>[2x]MKLYVFLVNTGTTLTFDTELTVQTVADLKHAIQSKYKIAIQHQVLVVNGGECMAADRRVCTYSAGTDTNPIFLFNKEMILCDRPPAIPKTTFSTENDMEIKVEESLMMPAVFHTVASRTQLALEMYEVAKKLCSFCEGLVHDEHLQHQGWAAIMANLEDCSNSYQKLLFKFESIYSNYLQSIEDIKLKLTHLGTAVSVMAKIPLLECLTRHSYRECLGRLDSLPEHEDSEKAEMKRSTELVLSPDMPRTTNESLLTSFPKSVEHVSPDTADAESGKEIRESCQSTVHQQDETTIDTKDGDLPFFNVSLLDWINVQDRPNDVESLVRKCFDSMSRLDPRIIRPFIAECRQTIAKLDNQNMKAIKGLEDRLYALDQMIASCGRLVNEQKELAQGFLANQKRAENLKDASVLPDLCLSHANQLMIMLQNHRKLLDIKQKCTTAKQELANNLHVRLKWCCFVMLHADQDGEKLQALLRLVIELLERVKIVEALSTVPQMYCLAVVEVVRRKMFIKHYREWAGALVKDGKRLYEAEKSKRESFGKLFRKSFLRNRLFRGLDSWPPSFCTQKPRKFDCELPDISLKDLQFLQSFCPSEVQPFLRVPLLCDFEPLHQHVLALHNLVKAAQSLDEMSQTITDLLSEQK;>MEQEHTEILRGLRFTLLFVQHVLEIAALKGSASEAAGGPEYQLQESVVADQISLLSREWGFAEQLVLYLKVAELLSSGLQSAIDQIRAGKLCLSSTVKQVVRRLNELYKASVVSCQGLSLRLQRFFLDKQRLLDRIHSITAERLIFSHAVQMVQSAALDEMFQHREGCVPRYHKALLLLEGLQHMLSDQADIENVTKCKLCIERRLSALLTGICA[2x];>[2x]HDVLETIFVRKVGAFVNKPINQVTLTSLDIPFAMFAPKNLELEDTDPMVNPPDSPETESPLQGSLHSDGSSGGSSGNTHDDFVMIDFKPAFSKDDILPMDLGTFYREFQNPPQLSSLSIDIGAQSMAEDLDSLPEKLAVHEKNVREFDAFVETLQ

The unc-51-like kinase protein kinase complex (ULK1C) and the class III phosphatidylinositol (PI) 3-kinase complex I (PI3KC3-C1) are the most upstream and central players in the initiation of macroautophagy. FIP200 is the central scaffolding subunit of the ULK1 complex (ULK1C), which also contains the ULK1 (or ULK2) kinase itself, ATG13, and ATG101. PI3KC3-C1 contains one copy each of the lipid kinase VPS34, the pseudokinase VPS15, and the regulatory subunits BECN1 and ATG14. The two complexes coassemble through extensive contacts between the FIP200 scaffold subunit of ULK1C and the VPS15 pseudokinase subunit of PI3KC3-C1.

ULK1C and PI3KC3-C1 were mixed and visualized by cryo-EM ([Fig figs6]). The presence of the ULK1^MIT^-ATG13^MIM^ heterodimer was confirmed on both of the FIP200 shoulders, demonstrating that the stoichiometry of the ULK1 complex is altered by the presence of PI3KC3-C1. The presence of PI3KC3-C1 induces a rearrangement of ULK1C from a FIP200:ATG13:ULK1 2:1:1 to a 2:2:2 stoichiometry by dislocating an ATG13 loop (ATG13^MR^) from an inhibitory site on the dimeric FIP200 scaffold. This suggests a mechanism for the initiation of autophagy through PI3KC3-C1-induced dimerization of ULK1 as bound to FIP200, followed by an activating trans-autophosphorylation of ULK1. The presence of an excess of 2:2:2 ULK1C cores relative to ULK1C: PI3KC3-C1 supercomplexes suggests that PI3KC3-C1 acts as an exchange factor to promote the 2:2:2 complex, serving to displace ATG13 from the autoinhibitory site #2. This model suggests that PI3KC3-C1 does not need to remain tightly bound in a supercomplex to ULK1C following activation, but PI3KC3-C1 would be susceptible to phosphorylation by ULK1 ^.>[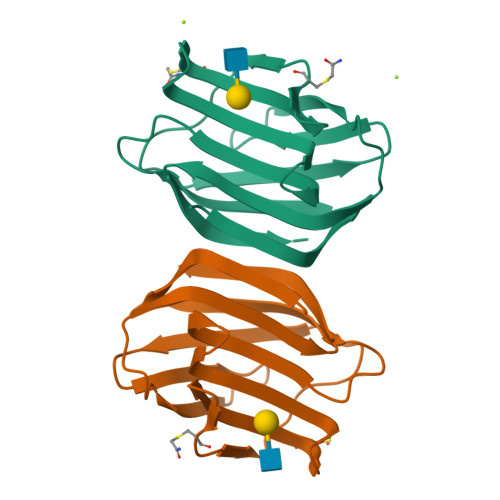2x]MAGVLIQNMSFKVGQTLTITGVPKPDSTNFAINIGHSPEDIALHMNPRFDAHGDQCTIVCNSFQSGSWCEEHRDDNFPFIQDKEFQIKITFTNEEFLVTLPDGSEIHFPNRQGSEKYKYMYFEGEVRIQGVEIK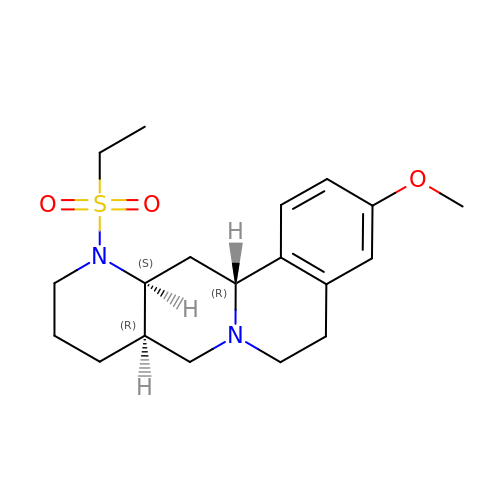(8~{a}~{R},12~{a}~{S},13~{a}~{R})-12-ethylsulfonyl-3-methoxy-5,6,8,8~{a},9,10,11,12~{a},13,13~{a}-decahydroisoquinolino[2,1-g][1,6]naphthyridine | C19 H28 N2 O3 S | UMGBFFAJXFXOIL-AYOQOUSVSA-N>[2x]AEEELPPRKVCIVGAGVSGLYIAMILDDLKIPNLTYDIFESSSRTGGRLYTHHFTDAKHDYYDIGAMRYPDIPSMKRTFNLFKRTGMPLIKYYLDGENTPQLYNNHFFAKGVVDPYMVSVANGGTVPDDVVDSVGEKLQQAFGYYKEKLAEDFDKGFDELMLVDDMTTREYLKRGGPKGEAPKYDFFAIQWMETQNTGTNLFDQAFSESVIASFDFDNPTKPEWYCIEGGTSLLVDAMKETLVHKVQNNKRVEAISIDLDAPDDGNMSVKIGGKD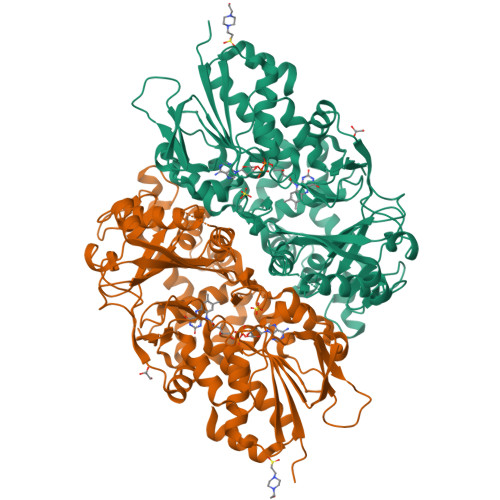YSGYSTVFNTTALGCLDRMDLRGLNLHPTQADAIRCLHYANSTKVALKFSYPWWIKDCGITCGGAASTDLPLRTCVYPSYNLGDTGEAVLLASYTWSQDATRIGSLVKDAPPQPPKEDELVELILQNLARLHAEHMTYEKIKEAYTGVYHAYCWANDPNVGGAFALFGPGQFSNLYPYLMRPAAGGKFHIVGEASSVHHAWIIGSLESAYTAVYQFLYKYKMWDYLRLLLERWQYGLQELETGKHGTAHLQFILGSLPKEYQVKI> GPHMKSPSAQELKEQGNRLFVGRKYPEAAACYGRAITRNPLVAVYYTNRALCYLKMQQPEQALADCRRALELDGQSVKAHFFLGQ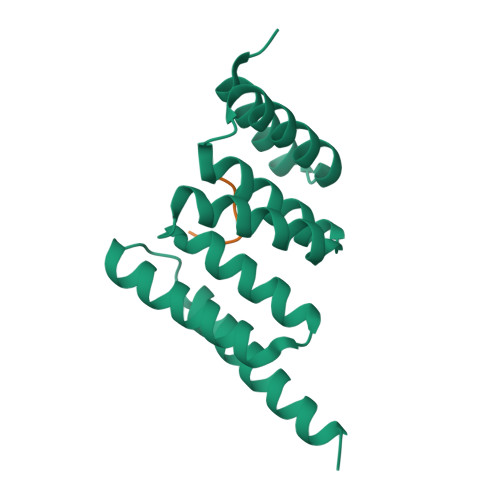CQLEMESYDEAIANLQRAYSLAKEQRLNFGDDIPSALRIAKKKRWNSIEERR;> GPTIEEVD> MHHHHHHSSRENLYFQGTLPLWIGKPGDKPPPLCGAIPASGDYVARPGDKVAARVKAVDGDEQWILAEVVSYSHATNKYEVDDIDEEGKERHTLSRRRVIPLPQWKANPETDPEALFQKE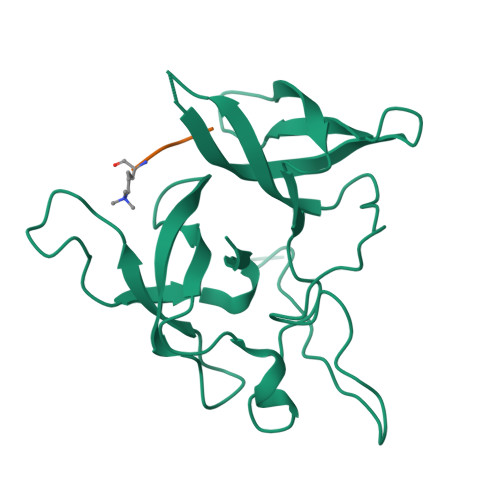QLVLALYPQTTCFYRALIHAPPQRPQDDYSVLFEDTSYADGYSPPLNVAQRYVVACKEPK;> ARTKQTARKST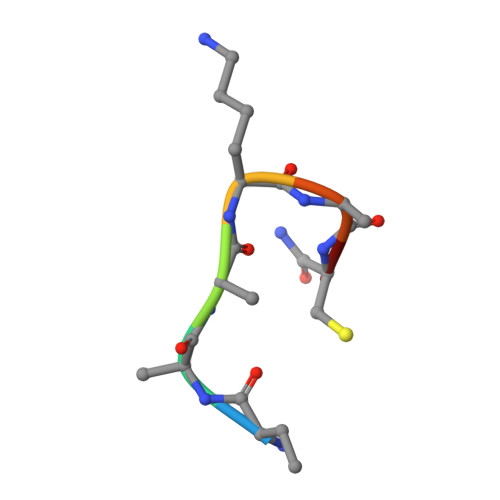> KAAKACX>[2x]MSVMYK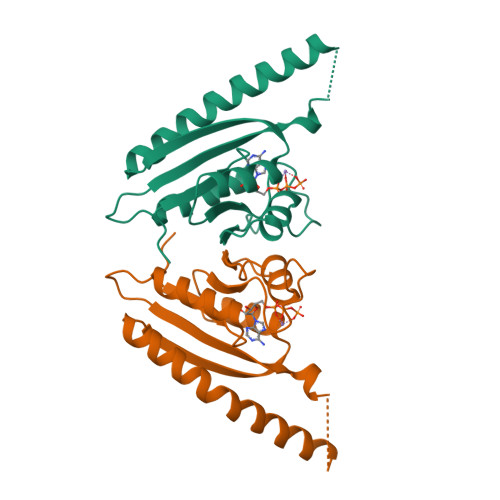KILYPTDFSETAEIALKHVKAFKTLKAEEVILLHVIDEREIKKRDIFSLLLGVAGLNKSVEEFENELKNKLTEEAKNKMENIKKELEDVGFKVKDIIVVGIPHEEIVKIAEDEGVDIIIMGSHGKTNLKEILLGSVTENVIKKSNKPVLVVKRKNS> MYDAIVVGGGFSGLKAARDLTNAGKKVLLLEGGERLGGRAYSRESRNVPGLRVEIGGAYLHRKHHPRLAAELDRYGIPTAAASEFTSFRHRLGPTAVDQAFPIPGSEAVAVEAATYTLLRDAHRIDLEKGLENQDLEDLDIPLNEYVDKLDLPPVSRQFLLAWAWNMLGQPADQASALWMLQLVAAHHYSILGVVLSLDEVFSNGSADLVDAMSQEIPEIRLQTVVTGIDQSGDVVNVTVKDGHAFQAHSVIVATPMNTWRRIVFTPALPERRRSVIEEGHGGQGLKILIHVRGAEAGIECVGDGIFPTLY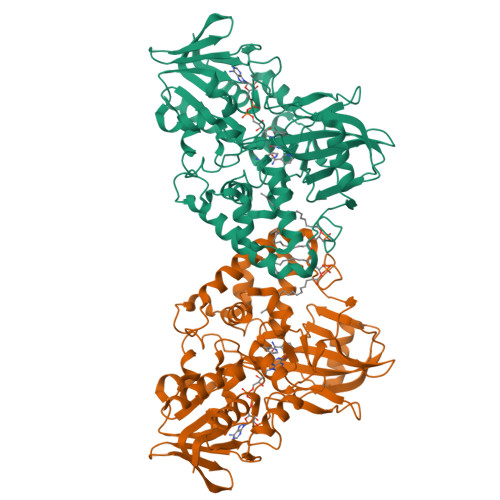DYCEVSESERLLVAFTDSGSFDPTDIGAVKDAVLYYLPEVEVLGIDYHDWIADPLFEGPWVAPRVGQFSRVHKELGEPAGRIHFVGSDVSLEFPGYIEGALETAECAVNAILHSHHHHHH> SKMDYDFKVKLSSERERVEDLFEYEGCKVGRGTYGHVYKAKRKDGKDDKDYALKQIEGTGISMSACREIALLRELKHPNVISLQKVFLSHADRKVWLLFDYAEHDLWHIIKFHRASKANKKPVQLPRGMVKSLLYQILDGIHYLHANWVLHRDLKPANILVMGEGPERGRVKIADMGFARLFNSPLKPLADLDPVVVTFWYRAPELLLGARHYTKAIDIWAIGCIFAELLTSEPIFHCRQEDIKTSNPYHHDQLDRIFNVMGFPADKDWEDIKKMPEHSTLMKDFRRNTYTNCSLIKYMEKHKVKPDSKAFHLLQKLLTMDPIKRITSEQAMQDPYFLEDPLPTSDVFAGCQIPYPKREFLTEEEPDDKGDKKNQQQQQGNNHTNGTGHPGNQDSSHTQGPPLKK;> KAMAGNFWQSSHYLQWILDKQDLLKERQKDLKFLSEEEYWKLQIFFTNVIQALGEHLKLRQQVIATATVYFKRFYARYSLKSIDPVLMAPTCVFLASKVEEFGVVSNTRLIAAATSVLKTRFSYAFPKEFPYRMNHILECEFYLLELMDCCLIVYHPYRPLLQYVQDMGQEDMLLPLAWRIVNDTYRTDLCLLYPPFMIALACLHVACVVQQKDARQWFAELSVDMEKILEIIRVILKLYEQWKNFDERKEMATILSKM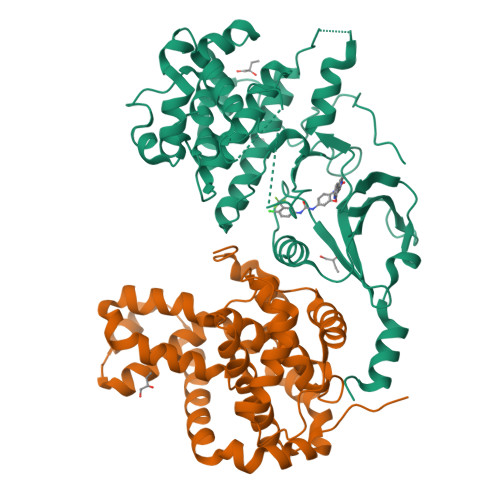PKPKPPPNSEGEQGPNGSQNSSYSQS>QELPQMTQQLNSDDMQEQLSATVKFRQILSREHRPPIDVVIQAGVVPRLVEFMRENQPEMLQLEAAWALTNIASGTSAQTKVVVDADAVPLFIQLLYTGSVEVKEQAIWALGNVAGDSTD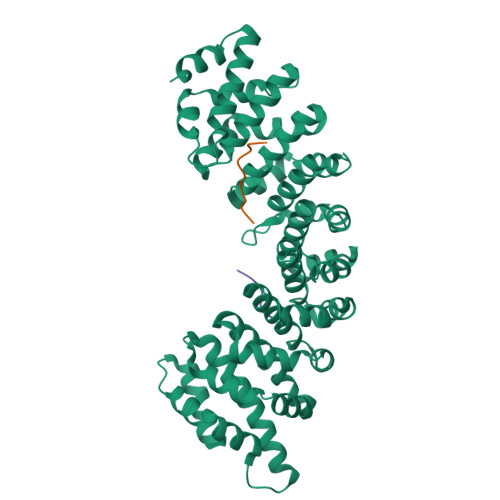YRDYVLQCNAMEPILGLFNSNKPSLIRTATWTLSNLCRGKKPQPDWSVVSQALPTLAKLIYSMDTETLVDACWAISYLSDGPQEAIQAVIDVRIPKRLVELLSHESTLVQTPALRAVGNIVTGNDLQTQVVINAGVLPALRLLLSSPKENIKKEACWTISNITAGNTEQIQAVIDANLIPPLVKLLEVAEDKTKKEACWAISNASSGGLQRPDIIRYLVSQGCIKPLCDLLEIADNRIIEVTLDALENILKMGEADKEARGLNINENADFIEKAGGMEKIFNCQQNENDKIYEKAYKIIETYF[2x];>PAAKRVKLD[4x]> MMSGAPSATQPATAETQHIADQVRSQLEEKYNKKFPVFKAVSFKSQVVAGTNYFIKVHVGDEDFVHLRVFQSLPHENKPLTLSNYQTNKAKHDELTY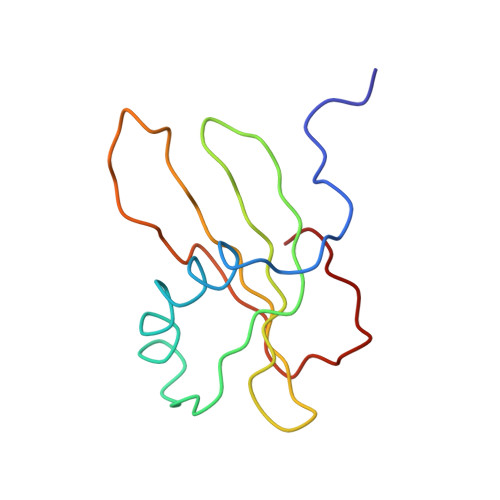F> GSDLTVSLIPVSG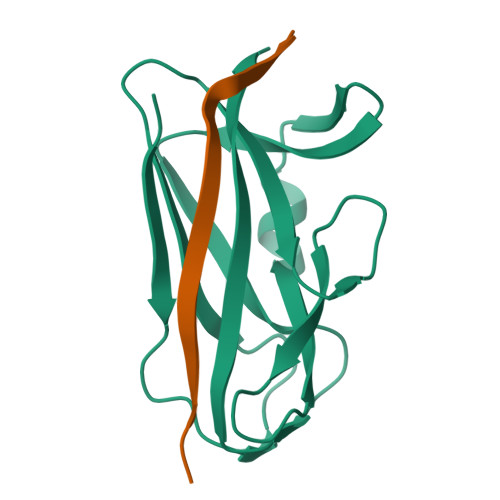LKAGKNAPSAKIAKLVVNSTTLKEFGVRGISNNVVDSTGTAWRVAGKNTGKEIGVGLSSDSLRRSDSTEKWNGVNWMTFNSNDTLDIVLTGPAQNVTADTYPITLDVVGYQP;> GSFLPNSEQQKSADIVFSSP> MAYEPQYYPGNTSVAQNRRKHMSGNVEKLREISDEDLTAILGHRAPGSDYPSTHPPLAEMGEPDCPIREIVEPTPGAAAGDRIRYVQWTDSMYNAPATPYWRSYYAAINHRGVDPGTLSGRQIVEARERDVEVYGKMSIETEMTCPALAGLRGATVHGHSCRLQE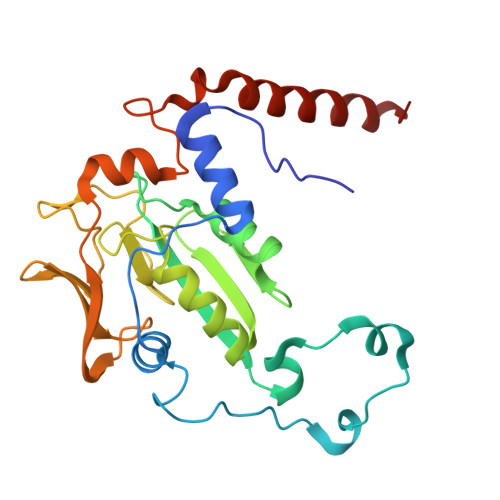DGVMFDMLDRRRLEGGTIIMDKDQVGVPLDRKVDLGKPMSEEEAAKRTTIYRVDNVPFRSDSEVVEWVQRIWELRTRYGFQPQ BCL-2 family proteins are crucial regulators of the mitochondrial apoptotic pathway and are characterized by the presence of up to four conserved BCL-2 Homology (BH) domains. BCL-2 family proteins are divided into 3 functionally distinct groups: (i) the pro-survival proteins (BCL-2, BCL-XL, BCL-W, MCL-1 and BFL-1/BCL2A1/A1), (ii) the multi-BH domain cell death effectors (BAX, BAK, BOK) and (iii) the BH3-only apoptosis initiators (e.g. BIM, BAD, NOXA). Dynamic interactions between members of BCL-2 family subgroups, involving binding of the BH3 domain of the pro-apoptotic members to a groove at the surface of the pro-survival proteins, control commitment to apoptosis. The pro-survival BCL-2 members exert their function by sequestering pro-apoptotic members through binding to their BH3 domains.

Here we describe S55746 (also known as BCL201), a novel, orally active BCL-2 specific inhibitor that has a partially overlapping but distinct BCL-2 hydrophobic groove binding mode compared to ABT-199. Fluorescence polarization (FP) data, using Fluorescent-PUMA as a binder, demonstrates that S55746 is a potent inhibitor of BCL-2 (Ki = 1.3 nM). The selectivity of S55746 for BCL-2 versus BCL-XL ranges from ~70 to 400 folds depending on the assay used. No significant binding to MCL-1 and BFL-1 was observed. S55746 occupies the region typically referred to as S1/2/3 in contrast to the ABT-199 analog, which occupies a greater portion of the protein surface area including S2/3/4/5. S55746 adopts essentially the same binding mode as described in Porter et al. 2009. S55746 forms a single hydrogen bond to the backbone carbonyl of residue A149 buried deep into S2. The size-independent enthalpic efficiency (0.83) for S55746 binding to BCL-2 is suggestive of optimal polar and Van der Waal's interactions, indicative of highly specific binding. Since ABT-199 and S55746 have different binding modes, one can theoretically speculate that mutation(s) in the BCL-2 protein could cause resistance to one compound and not the other. Altogether, these data demonstrate that S55746 kills cancer cells through on-target activity, meaning activation of a BAX/BAK-dependent mitochondrial apoptotic pathway by direct inhibition of the BCL-2 pro-survival protein.

> MHHHHHHHHLVPRGSYDNREIVMKYIHYKLSQRGYEWDAGADVEENRTEAPEGTESEVVHKTLREAGDDFSRRYRRDFAEMSSQLHLTPFTARGRFATVVEELFRDGVNWGRIVAFFEFGGVMCVESVNREMSPLVDNIALWMTEYLNRHLHTWIQDNGGWDAFVELYGPSM> SRPHQWQTDEEGVRTGKCSFPVKYLGHVEVDESRGMHICEDAVKRLKAERKFFKGFFGKTGKKAVKAVLWVSADGLRVVDEKTKDLIVDQTIEKVSFCAPDRNFDRAFSYICRDGTTRRWICHCFMAVKDTGERLS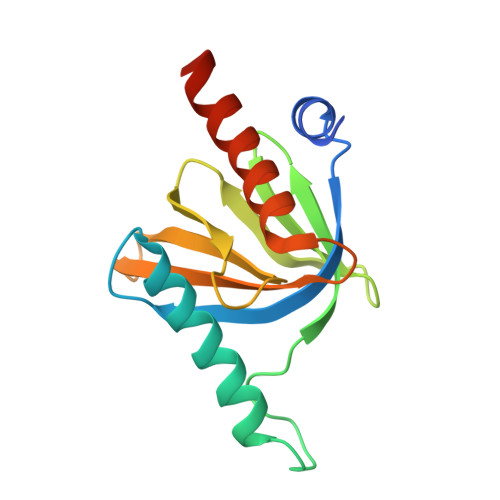HAVGCAFAACLERKQKREKE> MASMQKLINSVQNYAWGSKTALTELYGIANPQQQPMAELWMGAHPKSSSRITTANGETVSLRDAIEKNKTAMLGEAVANRFGELPFLFKVLCAAQPLSIQVHPNKRNSEIGFAKENAAGIPMDAAERNY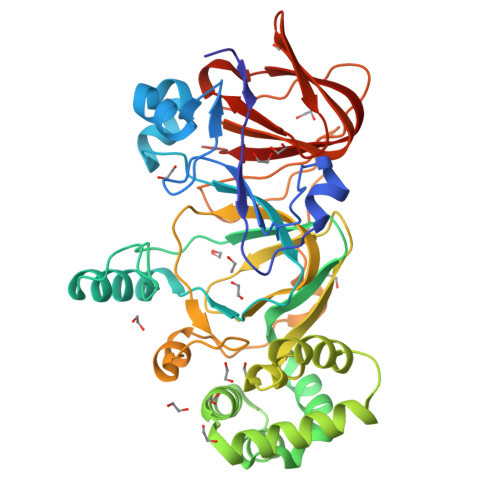KDPNHKPELVFALTPFLAMNAFREFSDIVSLLQPVAGAHSAIAHFLQVPNAERLSQLFASLLNMQGEEKSRALAVLKAALNSQQGEPWQTIRVISEYYPDDSGLFSPLLLNVVKLNPGEAMFLFAETPHAYLQGVALEVMANSDNVLRAGLTPKYIDIPELVANVKFEPKPAGELLTAPVKSGAELDFPIPVDDFAFSLHDLALQETSIGQHSAAILFCVEGEAVLRKDEQRLVLKPGESAFIGADESPVNASGTGRLARVYNKL> GVGLHFRGAEPWEEKIRAAAELGVTTVRLDATGPIEETVARIRAAAEAGITNLVLEPGPLALDELKAYRDAAPDTFLTVHIGDNPVLDDATIADIKAAGADAIGIPAKNIDDLIANLEKAK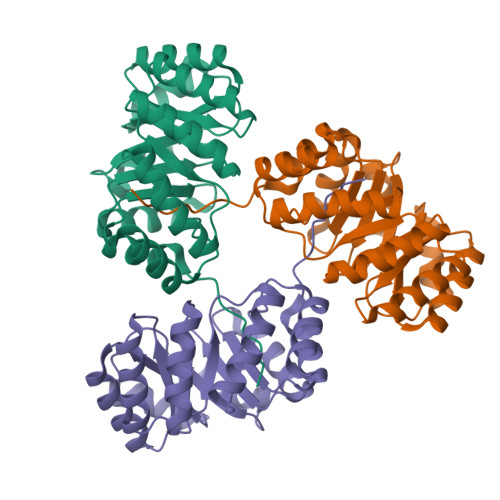AAGLKVLVGLLPGPKELVEEKVRAAAAAGAAALLLDLSDLEVAKAAIRVADEAGLPVLAGGGFDDVDSFVAAAEEIRALNPRATLLLEARGLATADIVAAMERALEHHHHHH4-AMINO-5-HYDROXYMETHYL-2-METHYLPYRIMIDINE | C6 H9 N3 O | 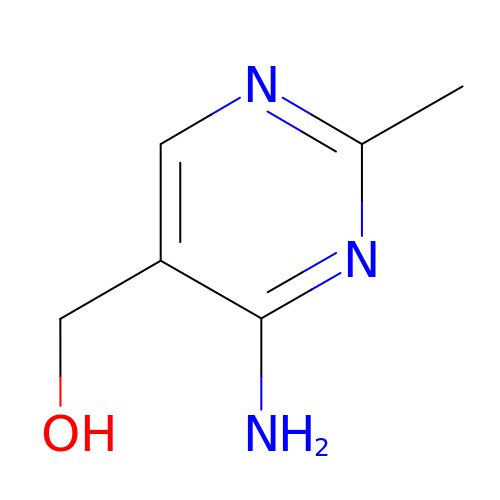VUTBELPREDJDDH-UHFFFAOYSA-N> MKTVVFAYHDMGCLGIEALLAAGYEISAIFTHTDNPGEKAFYGSVA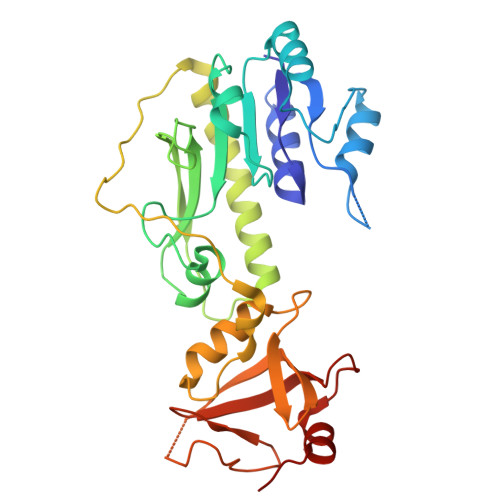RLAAERGIPVYAPDNVNHPLWVERIAQLSPDVIFSFYYRHLIYDEILQLAPAGAFNLHGSLLPKYRGRAPLNWVLVNGETETGVTLHRMVKRADAGAIVAQLRIAIAPDDIAITLHHKLCHAARQLLEQTLPAIKHGNILEIAQRENEATCFGRRTPDDSFLEWHKPASVLHNMVRAVADPWPGAFSYVGNQKFTVWSSRVHPHASKAQPGSVISVAPLLIACGDGALEIVTGQAGDGITMQGSQLAQTLGLVQ> MLYGGSRVQYLVQPPFTLHKIRSENLPPPSLYAERHDLGLEMQLPRDMHVYNSINMAIQRQVGGDSST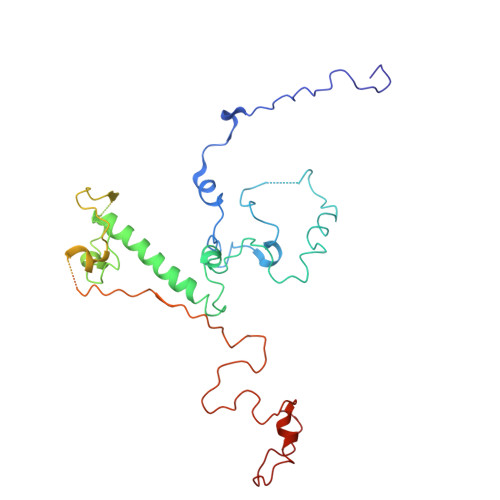LDGEQQQLQGGHADGFDMGAFFTEQHHPERHHNSSLPYAKHDTNNVLAMRLFPVNVGVRARTEAIRIRTDDCLQRLRDADLCAKMRLPLEHPLPLSRRSQYAAIHRVRQERCYDAPTEAAGERAAAAAEEASRTAHLRGAAAHPPPSELSIVTRPVDRLGSHSGSSAAACTADADHLSFPVHPFAAAAVSSGCHSARSGSAARLASQRWLPLQTLKPMGHNWSAATRSSGVRGPHMQLMQERLDQKGFGWKRKSRSLWQQDVATAGFRPHRYF(5S)-2-amino-3-methyl-5-pyridin-4-yl-5-(3-pyridin-3-ylphenyl)-3,5-dihydro-4H-imidazol-4-one | C20 H17 N5 O | 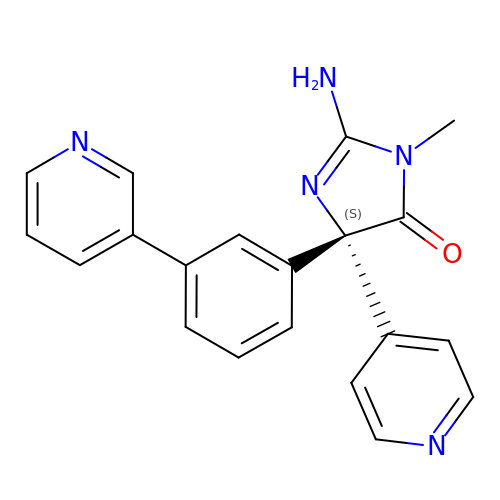AIKOTXHNUIYVMD-HXUWFJFHSA-N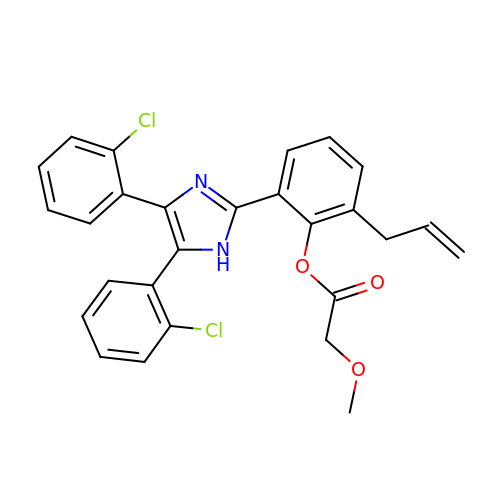2-[4,5-bis(2-chlorophenyl)-1H-imidazol-2-yl]-6-(prop-2-en-1-yl)phenyl methoxyacetate | C27 H22 Cl2 N2 O3 | XJUOIVVGPFMWJG-UHFFFAOYSA-N The proximal half-fiber is formed by a parallel homo-trimer of gp34. The protein is a highly intertwined trimer containing a 2 nm-wide triple β-helix domain interspersed with three wider domains in which each of the monomers forms an anti-parallel β-sheet. The long tail fibers recognize the outer membrane protein C (OmpC) or the lipopolysaccharide (LPS) of E. coli and are responsible for the initial and reversible attachment of the virion. The carboxy-terminal parts of gp34 that we crystallized occupy the part of the proximal tail fiber closest to gp35 (the “knee”).

The structure of gp34(894–1289) was determined using the single-wavelength anomalous dispersion method (SAD), using data from crystals of the P21 form grown from protein in which selenomethionine was incorporated. A high-multiplicity dataset measured to 2.0 Å resolution at the peak wavelength of selenium was collected and used for phase determination. Thirteen sites were found, where fifteen sites were expected (five internal methionines per monomer of the trimer). The resulting phases were of high quality and, after solvent flattening with 53.2% solvent, permitted automatic building of 1102 residues, of which 1095 were automatically docked into sequence. Manual fitting and refinement led to a final model consisting of 1189 residues (893–1288 of chain A, 893–1289 of chain B, and 893–1288 of chain C), plus seven glycerol molecules and 1620 water molecules (residue 893 is the final proline of the amino-terminal purification tag). Here, the refined model contained the same protein residues as before, plus seven glycerol molecules and 1312 water molecules. Both the native and selenomethionine-modified models have good correspondence to the measured data and reasonable stereochemical parameters, although residues at the amino- and carboxy-termini have higher temperature factors and show some disorder. Crystals belonging to two different space groups (P21 and R32) were obtained for gp34(894–1289).

>[3x]MGSSHHHHHHSQDPSQFIRRDIAQTVNGSLTLTQQTNLSAPLVSSSTGEFGGSLAANRTFTIRNTGAPTSIVFEKGPASGANPAQSMSIRVWGNQFGGGSDTTRSTVFEVGDDTSHHFYSQRNKDGNIAFNINGTVMPININASGLMNVNGTATFGRSVTANGEFISKSANAFRAINGDYGFFIRNDASNTYFLLTAAGDQTGGFNGLRPLLINNQSGQITIGEGLIIAKGVTINSGGLTVNSRIRSQGTKTSDLYTRAPTSDTVGFWSIDINDSATYNQFPGYFKMVEKTNEVTGLPYLERGEEVKSPGTLTQFGNTLDSLYQDWITYPTTPEARTTRWTRTWQKTKNSWSSFVQVFDGGNPPQPSDIGALPSDNATMGNLTIRDFLRIGNVRIVPDPVNKTVKFEWVE4-[(dimethylamino)methyl]benzonitrile | C10 H12 N2 | 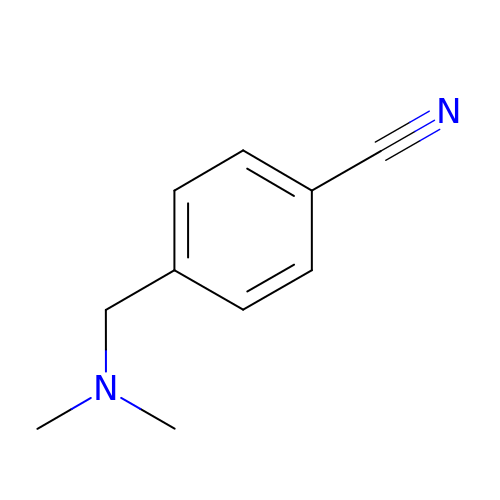QCSOEUMGZOKXPJ-UHFFFAOYSA-N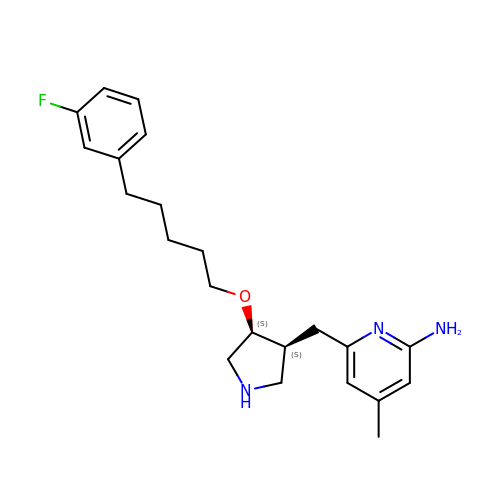6-{[(3S,4S)-4-{[5-(3-fluorophenyl)pentyl]oxy}pyrrolidin-3-yl]methyl}-4-methylpyridin-2-amine | C22 H30 F N3 O | AQTALODLFZOZJL-GHTZIAJQSA-N> MIDLREDTWTLQLYAQRYKGLSPKNSRELQLRMEYDPLKPNLPTSGEEQNSKPEWLNTPPCLIPESESLDKAKGALVGLAIGDAIGTTLEFLPRDKLHVNDMVGGGPFRLQPGEWTDDTSMALCLAESYISAGRLDITLFREKLVRWYRHGENSSNGRCFDIGNTTRNALEQYLKHGASWFGNTEPETAGNAAIIRQAPTSIFRRKSLQRTFADSDSQSMATHCAPESMASCQFLGFILNYLINGSSREKAFSPHVMPLPVRVLLINAGEYKEKKRDEIRSSGYVIDTLEAAMWAVWNTDNFHDAILLAANLGDDADSVA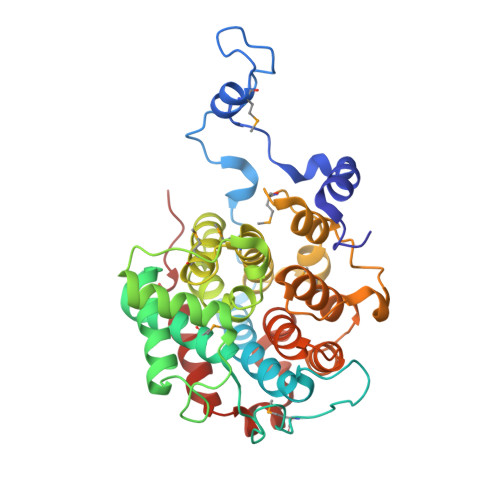ATTGQIAGALYGYSNIPKPWLDKLVQQERISNLAEQLFYMAPEEDF>[2x]MHHHHHHMAGMLTVGDLVIEESTYTARLKGRALELTYKEFELLKYLAQHAGRVFTRAQLLQEVWGYDFFGGTRTVDVHVRRLRAKLGPEYDSMIGTVRNVGYKFVRPSR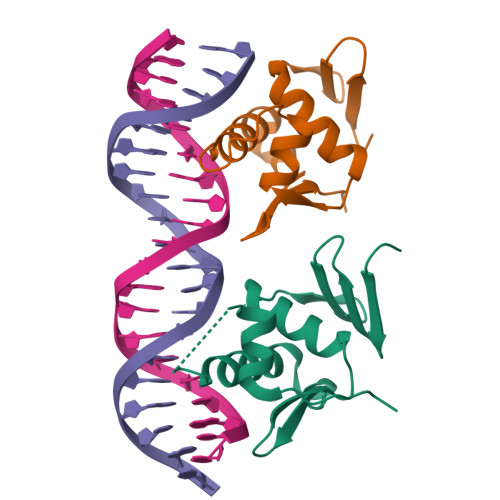SSQPASPIVAEERQDAATQADAPAQRSAESAVVR> GSHMASLKDLEGKWRLMESHGFEEY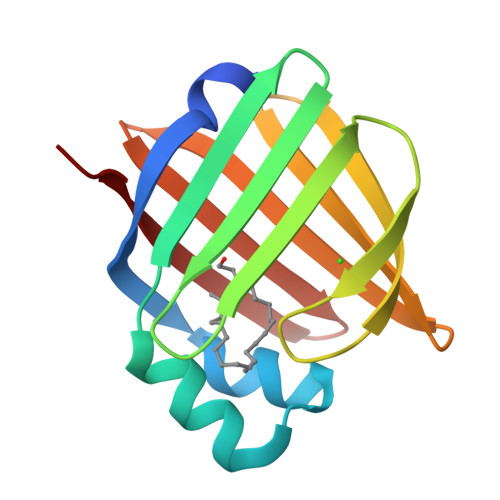MKELGVGLALRKMAAMAKPDCIITCDGNNITVKTESTVKTTVFSCNLGEKFDETTADGRKTETVCTFQDGALVQHQQWDGKESTITRKLKDGKMIVECVMNNATCTRVYEKVQ>QGPAMGYARRVMDGIGEVAVTGAGGSVTGARLRHQVRLLAHALTEAGIPPGRGVACLHANTWRAIALRLAVQAIGCHYVGLRPTAAVTEQARAIAAADSAALVFEPSVEARAADLLERVSVPVVLSLGPTSRGRDILAASVPEGTPLRYREHPEGIAVVAFTSGTTGTPKGVAHSSTAMSACVDAAVSMYGRGPWRFLIPIPLSDLGGELAQCTLATGGTVVLLEEFQPDAVLEAIERERATHVFLAPNWLYQLAEHPALPRSDLSSLRRVVY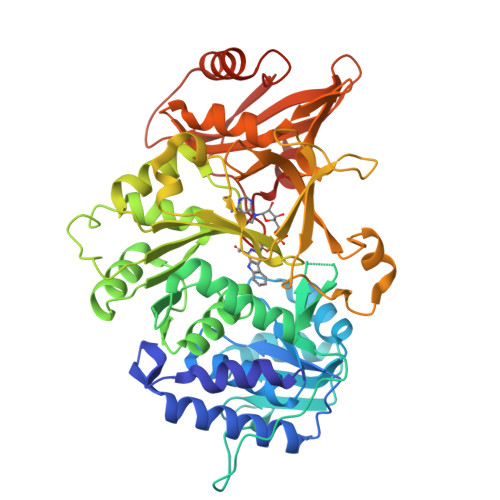GGAPAVPSRVAAARERMGAVLMQNYGTQEAAFIAALTPDDHARRELLTAVGRPLPHVEVEIRDDSGGTLPRGAVGEVWVRSPMTMSGYWRDPERTAQVLSGGWLRTGDVGTFDEDGHLHLTDRLQDIIIVEAYNVYSRRVEHVLTEHPDVRAAAVVGVPDPDSGEAVCAAVVVADGADPDPEHLRALVRDHLGDLHVPRRVEFVRSIPVTPAGAPDKVKVRTWFTD[5x]> SNASAATVDLRVLETTDLHSNMMDFDYYKDKPTEKFGLVRTASLIIAARQQATNSVLVDNGDVIQGSPLGDYIAAKGLNDGEIHPVYKAMNTLDYAVGNIGNHEFNYGLDYLKKSLAGAKFPYVNANVIDVKTGKPLFQPYLIIDTPVKDRDGKSHNLRIGYIGFVPPQVMIWDKANL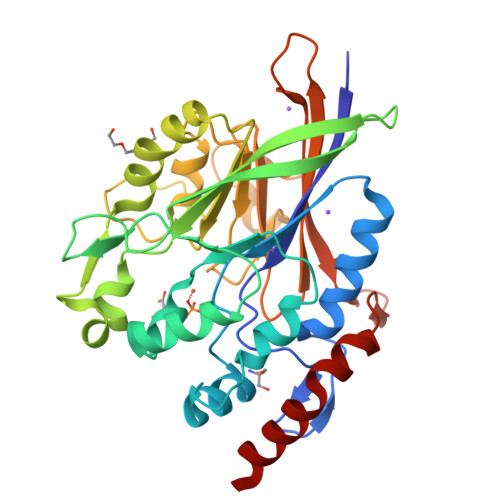SGKVTVNDITETAKKWVPEMREQGADLVVAIPHSGLSSDPYKTMAENSVYYLSQVPGIDAIMFGHAHGVFPSKDFAAIKGADITQGTLNGIPAVMPGQWGDHLGVVDFVLNNDQGKWQVIDAKAEARPIYDKTAQKSLAAENAKLVEVLAVDHQSTRDFVSQ>MEDINFSSLAPRHGTRPFMGTWSDIGTSQLNGGAFNWSSLWSGLKNFGSTLKTYGSKAWNSTTGQALRDKLKEQNFQQKVVDGLASGINGVVDLANQAVQRQINSRLDPVPPAGSVEMPQVEEELPPLDKRGEKRPRPDAEETLLTHTDEPPPYEEAVKLGLPTTRPIAPLATGVLKPESNKPATLDLPPPASRPSTVAKPLPPVAVARARPGGSARPHANWQSTLNSIVGLGVQSVKRRRCY[12x];>[12x]MATPSMLPQWAYMHIAGQDASEYLSPGLVQFARATDTYFSLGNKFRNPTVAPTHDVTTDRSQRLTLRFVPVDREDNTYSYKVRYTLAVGDNRVLDMASTYFDIRGVLDRGPSFKPYSGTAYNSLAPKGAPNSSQWEQKKAGNGDTMETHTFGVAPMGGENITIDGLQIGTDATADQDKPIYADKTFQPEPQVGEENWQETESFYGGRALKKDTSMKPCYGSYARPTNVKGGQAKLKVGADGVPTKEFDIDLAFFDTPGGTVNGQDEYKADIVMYTENTYLETPDTHVVYKPGKDDASSEINLVQQSMPNRPNYIGFRDNFIGLMYYNSTGNMGVLAGQASQLNAVVDLQDRNTELSYQLLLDSLGDRTRYFSMWNQAVDSYDPDVRIIENHGVEDELPNYCFPLDGSGTNAAYQGVKVKNGNDGDVESEWENDDTVAARNQLCKGNIFAMEINLQANLWRSFLYSNVALYLPDSYKYTPANITLPTNTNTYDYMNGRVVPPSLVDAYINIGARWSLDPMDNVNPFNHHRNAGLRYRSMLLGNGRYVPFHIQVPQKFFAIKSLLLLPGSYTYEWNFRKDVNMILQSSLGNDLRTDGASISFTSINLYATFFPMAHNTASTLEAMLRNDTNDQSFNDYLSAANMLYPIPANATNVPISIPSRNWAAFRGWSFTRLKTKETPSLGSGFDPYFVYSGSIPYLDGTFYLNHTFKKVSITFDSSVSWPGNDRLLTPNEFEIKRTVDGEGYNVAQCNMTKDWFLVQMLAHYNIGYQGFYVPEGYKDRMYSFFRNFQPMSRQVVDEVNYKDYQAVTLAYQHNNSGFVGYLAPTMRQGQPYPANYPYPLIGKSAVTSVTQKKFLCDRVMWRIPFSSNFMSMGALTDLGQNMLYANSAHALDMNFEVDPMDESTLLYVVFEVFDVVRVHQPHRGVIEAVYLRTPFSAGNATT;> MMRRAYPEGPPPSYESVMQQAMAAAAAMQPPLEAPYVPPRYLAPTEGRNSIRYSELAPLYDTTRLYLVDNKSADIASLNYQNDHSNFLTTVVQNNDFTPTEASTQTINFDERSRWGGQLKTIMHTNMPNVNEFMYSNKFKARVMVSRKTPNGVTVTDGSQDILEYEWVEFELPEGNFSVTMTIDLMNNAIIDNYLAVGRQNGVLESDIGVKFDTRNFRLGWDPVTELVMPGVYTNEAFHPDIVLLPGCGVDFTESRLSNLLGIRKRQPFQEGFQIMYEDLEGGNIPALLDVDAYEKSKEESAAAATAAVATASTEVRGDNFASPAAVAAAEAAETESKIVIQPVEKDSKDRSYNVLPDKINTAYRSWYLAYNYGDPEKGVRSWTLLTTSDVTCGVEQVYWSLPDMMQDPVTFRSTRQVSNYPVVGAELLPVYSKSFFNEQAVYSQQLRAFTSLTHVFNRFPENQILVRPPAPTITTVSENVPALTDHGTLPLRSSIRGVQRVTVTDARRRTCPYVYKALGIVAPRVLSSRTF;>MSGSGSFEGGVFSPYLTGRLPSWAGVRQNVMGSTVDGRPVQPANSSTLTYATLSSSSVDAAAAAAAASAASAVRGMAMGAGYYGTLVANSSSTNNPASLNEEKLLLLMAQLEALTQRLGELTQQVAQLQEQTRAAVATVKSK[4x];> MQQQPPPDPAMRAALQSQPSGINSSDDWTQAMQRIMALTTRNPEAFRQQPQANRLSAILEAVVPSRSNPTHEKVLAIVNALVENKAIRGDEAGLVYNALLERVARYNSTNVQTNLDRMVTDVREAVAQRERFHRESNLGSMVALNAFLSTQPANVPRGQEDYTNFISALRLMVTEVPQSEVYQSGPDYFFQTSRQGLQTVNLSQAFKNLQGLWGVQAPVGDRATVSSLLTPNSRLLLLLVAPFTDSGSINRNSYLGYLINLYREAIGQAHVDEQTYQEITHVSRALGQDDPGNLEATLNFLLTNRSQKIPPQYTLSAEEERILRYVQQSVGLFLMQEGATPSAA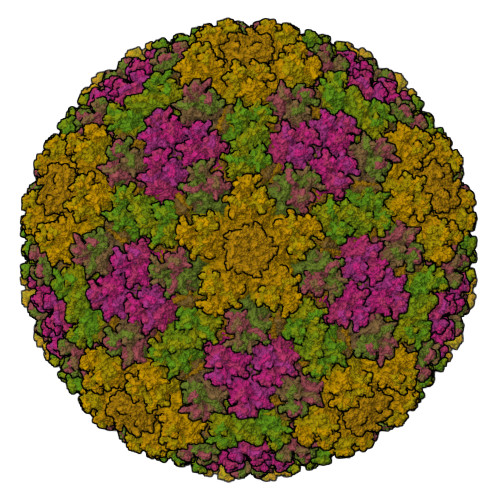LDMTARNMEPSMYASNRPFINKLMDYLHRAAAMNSDYFTNAILNPHWLPPPGFYTGEYDMPDPNDGFLWDDVDSSVFSPRPGANERPLWKKEGSDRRPSSALSGREGAAAAVPEAASPFPSLPFSLNSIRSSELGRITRPRLLGEEEYLNDSLLRPEREKNFPNNGIESLVDKMSRWKTYAQEHRDDPSQGATSRGSAARKRRWHDRQRGLMWDDEDSADDSSVLDLGGSGNPFAHLRPRIGRMM;>MSKEIPTPYMWSYQPQMGLAAGAAQDYSTRMNWLSAGPAMISRVNDIRAHRNQILLEQSALTATPRNHLNPRNWPAALVYQEIPQPTTVLLPRDAQAEVQLTNSGVQLAGGATLCRHRPAQGIKRLVIRGRGTQLNDEVVSSSLGLRPDGVFQLAGSGRSSFTPRQAVLTLESSSSQPRSGGIGTLQFVEEFTPSVYFNPFSGSPGHYPDEFIPNFDAISESVDGYD[2x]Sirtuins (SIRTs) are nicotinamide adenine dinucleotide (NAD+)‐dependent lysine deacylases linked to key physiological and disease processes. SIRTs catalyze lysine deacylation through a distinctive mechanism in which the amide oxygen of the acylated lysine transiently attacks the C1’ of the nicotinamide riboside residue from NAD+ (hereafter referred to as C1’ of NAD+ ribose), forming a covalent ADP‐ribosylated intermediate. Here, we report a new class of mechanism‐based 1,2,3‐triazole inhibitors that hijack SIRT catalysis by forming stalled triazolium– or triazole–ADP‐ribose (ADPR) adducts derived from the cofactor NAD+. These trapped adducts inhibit the enzyme without covalent protein modification, prompting us to term the compounds “Sirtuin Trapping Ligands” (SirTraps).

To determine isoform selectivity, all compounds were tested against SIRT1 and SIRT3, the closest SIRT2 homologs. Accordingly, most compounds inhibited SIRT1 and SIRT3 deacetylation with nanomolar affinity. Superimposition with SIRT2–[6–ADPR] revealed a highly conserved binding mode, in which 6–ADPR maintains key interactions with His248 and Gln228, corresponding to His187 and Gln167 in SIRT2.

> GHMSDKGKLSLQDVAELIRARACQRVVVMVGAGISTPSGIPDFRSPGSGLYSNLQQYDLPYPEAIFELPFFFHNPKPFFTLAKELYPGNYKPNVTHYFLRLLHDKGLLLRLYTQNIDGLERVSGIPASKLVEAHGTFASATCTVCQRPFPGEDIRADVMADRVPRCPVCTGVVKPDIVFFGEPLPQRFLLHVVDFPMADLLLILGTSLEVEPFASLTEAVRSSVPRLLINRDLVGPLAWHPRSRDVAQLGDVVHGVESLVELLGWTEEMRDLVQRETGKLD;> EALPKATGG> MKLDIKKTFSNRSDRVKGIDFHPTEPWVLTTLYSGRVEIWNYETQVEVRSIQVTETPVRAGKFIARKNWIIVGSDDFRIRVFNYNTGEKVVDFEAHPDYIRSIAVHPTKPYVLSGSDDLTVKLWNWENNWALEQTFEGHEHFVMCVAFNPKDPSTFAS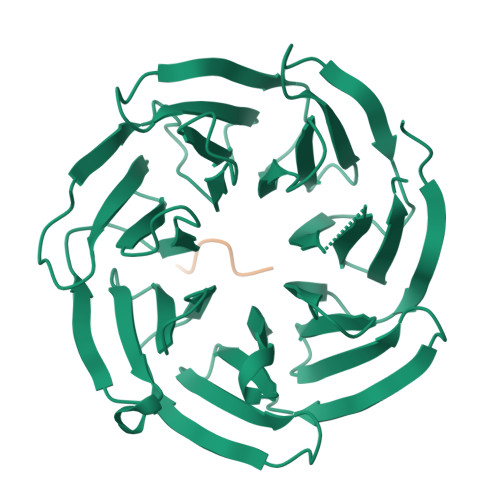GCLDRTVKVWSLGQSTPNFTLTTGQERGVNYVDYYPLPDKPYMITASDDLTIKIWDYQTKSCVATLEGHMSNVSFAVFHPTLPIIISGSEDGTLKIWNSSTYKVEKTLNVGLERSWCIATHPTGRKNYIASGFDNGFTVLSLG;> VKLHYT>[52x]MNNLYRDLAPVTEAAWAEIELEAARTFKRHIAGRRVVDVSDPGGPVTAAVSTGRLIDVKAPTNGVIAHLRASKPLVRLRVPFTLSRNEIDDVERGSKDSDWEPVKEAAKKLAFVEDRTIFEGYSAASIEGIRSASSNPALTLPEDPREIPDVISQALSELRLAGVDGPYSVLLSADVYTKVSETSDHGYPIREHLNRLVDGDIIWAPAIDGAFVLTTRGGDFDLQLGTDVAIGYASHDTDTVRLYLQETLTFLCYTAEASVALSH

Encapsulins are a class of BMCs characterised by their conserved subunit (Enc), which self-assembles to encapsulate enzymatically active cargoes and can remain porous to cargo substrates. The overall structure of Enc subunits across species with different T numbers is conserved and consists of a peripheral domain (P-domain), an axial domain (A-domain), and an extension loop (E-loop). T = 1 encapsulins of Mycobacterium tuberculosis, the causative agent of tuberculosis, and the closely related Mycobacterium marinum, are known to encapsulate the DyP as a core cargo with iron storage ferritin protein (BfrB)28 and FolB as possible secondary cargoes. In vitro cryo-electron microscopy (EM) single-particle analysis of the Mycobacterium tuberculosis encapsulin was used to obtain three structures of the encapsulin shell in intermediate states, as well as a 2.3 Å structure of the fully assembled shell.

In addition, we studied partial encapsulin structures to characterise stable encapsulin shell intermediates in vitro, by using low pH conditions to disassemble encapsulin shells, followed by reassembly at neutral pH. To explore the structural landscape of encapsulin shell formation, we used 2D and 3D (focused) classification and local symmetry to determine the structure of different stable encapsulin intermediates in an incomplete assembly state. This resulted in structures of three distinct intermediates of the encapsulin shell; a 48-mer (3,427 particles, 5.4 Å), a 52-mer (4,378 particles, 4.5 Å) and a 54-mer (6,294 particles, 4.6 Å). All three intermediates have an even number of monomers, appear to be closed on one side of the shell, and miss subunits on the other end. All three stable intermediates have an overall icosahedral structure with RMSD values for the 48,52 and 54-mer compared to the structure of the full shell of 1.08 Å, 0.60 Å and 2.66 Å respectively, although the 54-mer is, compared to the full encapsulin, flattened in one direction and elongated perpendicularly to it. The 52-mer consists of 39 fully resolved, and 13 less well resolved monomers, and the 54-mer consists of 27 fully resolved monomers and 27 less well resolved monomers. The 48-mer and the 52-mer differ primarily by the addition of two more Enctb dimers along the edge, around a point of threefold symmetry. The addition of these dimers appears to increase the stability of Enctb subunits that previously were located directly on the edge of the hole. Based on the predicted positive ΔG for Enc-Enc binding within pentamers, inclusion of dimers or pairs of monomers around trimers could be more prominent in driving these reactions. This would be consistent with the experimental structures obtained of 48- and 52-mer encapsulin shells, which differ by the addition of two dimers around a point of 3-fold symmetry as well the multimer Alphafold predictions, which predicts the inclusion of dimers around points of threefold symmetry.> AATPAAVTCQLSNWSEWTDCFPCQDKKYRHRSLLQPNKFGGTICSGDIWDQASCSSSTTCVRQAQCGQDFQCKETGRCLKRHLVCNGDQDCLDGSDEDDCEDVRAIDEDCSQYEPIPGSQKAALGYNILTQEDAQSVYDASYYGGQCETVYNGEWRELRYDSTCERLYYGDDEKYFRKPYNFLKYHFEALADTGISSEFYDNANDLLSKVKKDKSDSFGVTIGIGPAGSPLLVGVGVSHSQDTSFLNELNKYNEKKFIFTRI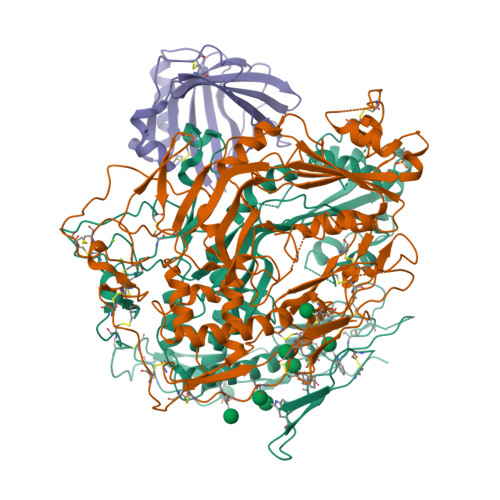FTKVQTAHFKMRKDDIMLDEGMLQSLMELPDQYNYGMYAKFINDYGTHYITSGSMGGIYEYILVIDKAKMESLGITSRDITTCFGGSLGIQYEDKINVGGGLSGDHCKKFGGGKTERARKAMAVEDIISRVRGGSSGWSGGLAQNRSTITYRSWGRSLKYNPVVIDFEMQPIHEVLRHTSLGPLEAKRQNLRRALDQYLMEFNACRCGPCFNNGVPILEGTSCRCQCRLGSLGAACEQTQTEGAKADGSWSCWSSWSVCRAGIQERRRECDNPAPQNGGASCPGRKVQTQAC;> SVDVTLMPIDCELSSWSSWTTCDPCQKKRYRYAYLLQPSQFHGEPCNFSDKEVEDCVTNRPCRSQVRCEGFVCAQTGRCVNRRLLCNGDNDCGDQSDEANCRRIYKKCQHEMDQYWGIGSLASGINLFTNSFEGPVLDHRYYAGGCSPHYILNTRFRKPYNVESYTPQTQGKYEFILKEYESYSDFERNVTEKMASKSGFSFGFKIPGIFELGISSQSDRGKHYIRRTKRFSHTKSVFLHARSDLEVAHYKLKPRSLMLHYEFLQRVKRLPLEYSYGEYRDLFRDFGTHYITEAVLGGIYEYTLVMNKEAMERGDYTLNNVHACAKNDFKIGGAIEEVYVSLGVSVGKCRGILNEIKDRNKRDTMVEDLVVLVRGGASEHITTLAYQELPTADLMQEWGDAVQYNPAIIKVKVEPLYELVTATDFAYSSTVRQNMKQALEEFQKEVSSCHCAPCQGNGVPVLKGSRCDCICPVGSQGLACEVSYRKNTPIDGKWNCWSNWSSCSGRRKTRQRQCNNPPPQNGGSPCSGPASETLDCS;> QKPQRPRRPASPISTIQPKANFDAQQFAGTWLLVAVGSACRFLQEQGHRAEATTLHVAPQGTAMAVSTFRKLDGICWQVRQLYGDTGVLGRFLLQARDARGAVHVVVAETDYQSFAVLYLERAGQLSVKLYARSLPVSDSVLSGFEQRVQEAHLTEDQIFYFPKYGFCEAADQFHVLDEVRR>G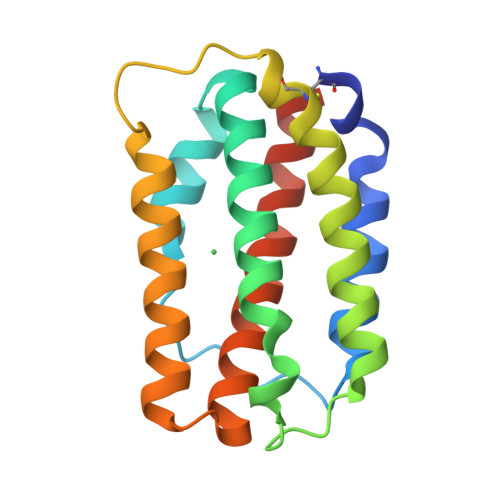STCEWLGRYRIITTESLNLLKNMGGKYADLETPFPSRLYTLMDKSKVEDQVKFLVLTLDHIIHLMDAREHMNSVNWDQNTVEDFLNILHRKSSDLKECVARYAKPAHKESYEIRIKRHFRTLKKILKKKQYSAEAWEQIRRVVKSHLQRMDIIASNARVNPRV[2x]>[2x]MHHHHHHSDKLLLSPAELLAHWQGHRDLTRRVIEAFPEEGFAAHHAPDMRPFQAMACELAGMVEYQLDWFRRGQPTWDENDQKKELPGRAELLAWWDKLTA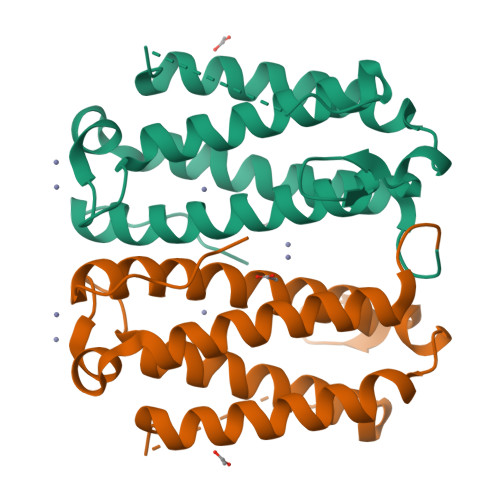ELGAEVPQVSTEMWATPATTPFGKMSPLMSVMYLIDNEVHHRGQGYVYLRELGVTPPAFYERRNLPPLG>MANLLKTVVTGCSCPFLSNLGSCKVLPGKKNFLRTFHTHRILWCKAPVKPGIPYKQLTVGVPKEIFQNEKRVALSPAGVQALVKQGFNVVVESGAGEASKFSDDHYRAAGAQIQGAKEVLASDLVVKVRAPMLNPTLGIHEADLLKTSGTLISFIYPAQNPDLLNKLSKRNTTVLAMDQVPRVTIAQGYDALSSMANIAGYKAVVLAANHFGRFFTGQITAAGKVPPAKILIVGGGVAGLASAGAAKSMGAIVRGFDTRAAALEQFKSLGAEPLEVDLKESGEGQGGYAKEMSKEFIEAEMKLFAQQCKEVDILISTALIPGKKAPILFNKEMIESMKEGSVVVDLAAEAGGNFETTKPGELYVHKGITHIGYTDLPSRMATQASTLYSNNITKLLKAISPDKDNFYFEVKDDFDFGTMGHVIRGTVVMKDGQVIFPAPTPKNIPQGAPVKQKTVAELEAEKAATITPFRKTMTSASVYTAGLTGILGLGIAAPNLAFSQMVTTFGLAGIVGYHTVWGVTPALHSPLM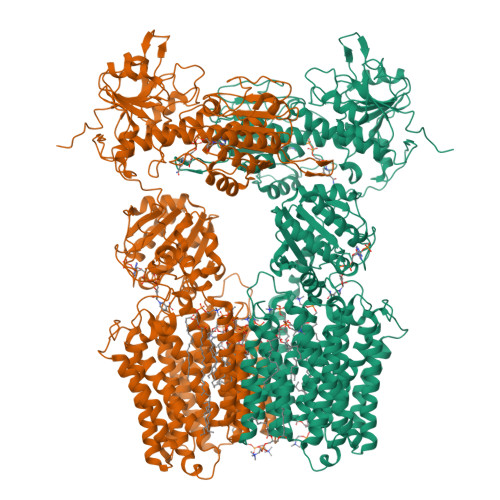SVTNAISGLTAVGGLVLMGGHLYPSTTSQGLAALATFISSVNIAGGFLVTQRMLDMFKRPTDPPEYNYLYLLPAGTFVGGYLASLYSGYNIEQIMYLGSGLCCVGALAGLSTQGTARLGNALGMIGVAGGLAATLGGLKPCPELLAQMSGAMALGGTIGLTIAKRIQISDLPQLVAAFHSLVGLAAVLTCIAEYIIEYPHFATDAAANLTKIVAYLGTYIGGVTFSGSLVAYGKLQGILKSAPLLLPGRHLLNAGLLAASVGGIIPFMMDPSFTTGITCLGSVSALSAVMGVTLTAAIGGADMPVVITVLNSYSGWALCAEGFLLNNNLLTIVGALIGSSGAILSYIMCVAMNRSLANVILGGYGTTSTAGGKPMEISGTHTEINLDNAIDMIREANSIIITPGYGLCAAKAQYPIADLVKMLSEQGKKVRFGIHPVAGRMPGQLNVLLAEAGVPYDIVLEMDEINHDFPDTDLVLVIGANDTVNSAAQEDPNSIIAGMPVLEVWKSKQVIVMKRSLGVGYAAVDNPIFYKPNTAMLLGDAKKTCDALQAKVRESYQK[2x]>MGSSHHHHHHLVPRGSHMMSQERRNPFLFKSNKFLTLFENENGHIRLLQRFDKRSDLFENLQNYRLVEY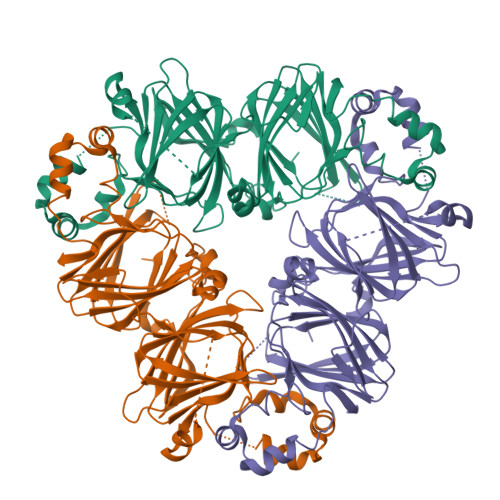RAKPHTIFLPQHIDADLILVVLSGKAILTVLSPNDRNSYNLERGDTIKLPAGTTSYLVNQDDEEDLRLVDLVIPVNGPGKFEAFDLAKNKNQYLRGFSKNILEASYNTRYETIEKVLLEEQEKDRKRRQQGEETDAIVKVSREQIEELKKLAKSSSKKSLPSEFEPINLRSHKPEYSNKFGKLFEITPEKKYPQLQDLDLFVSCVEINEGALMLPHYNSRAIVVLLVNEGKGNLELLGLKNEQQEREDRKERNNEVQRYEARLSPGDVVIIPAGHPVAITASSNLNLLGFGINAENNERNFLSGSDDNVISQIENPVKELTFPGSVQEINRLIKNQKQSHFANA[3x]> MGHHHHHHMVSQETIKHVKDLIAENEIFVA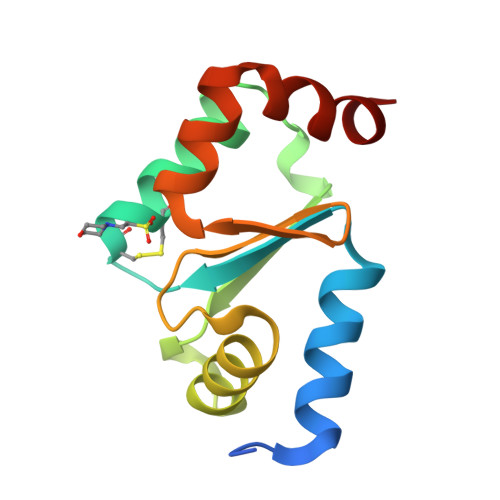SKTYCPYCHAALNTLFEKLKVPRSKVLVLQLNDMKEGADIQAALYEINGQRTVPNIYINGKHIGGNDDLQELRETGELEELLEPILAN>ETGFVNKDQIAKDVKQFYDQALQQAVVDDDANNAKAVVKTFHETLDCCGSSTLTALTTSVLKNNLCPSGSNIISNLFK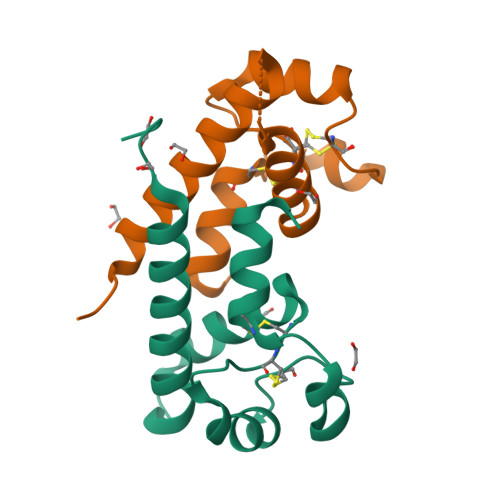EDCHQKIDDLFSGKGTKHHHHHH[2x]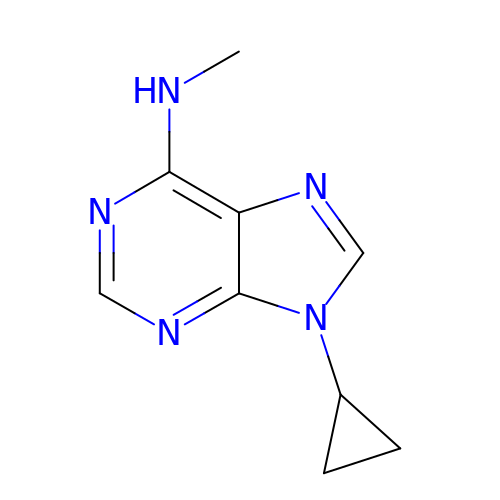9-cyclopropyl-~{N}-methyl-purin-6-amine | C9 H11 N5 | GSKXLJNKAAXSOE-UHFFFAOYSA-N>ALGVPFFSCQRGYKGVWRGDGIMQTTCPCGAQITGHVKNGSMRIVGPRTCSNTWHGTFPINAYTTGPCTPSPAPNYSRALWRVAAEEYVEVTRVGDFHYVTGMTTDNVKCPCQVPAPEFFTEVDGVRLHRYAPACKPLLREEVTFLVGLNQYLVGSQLPCEPEP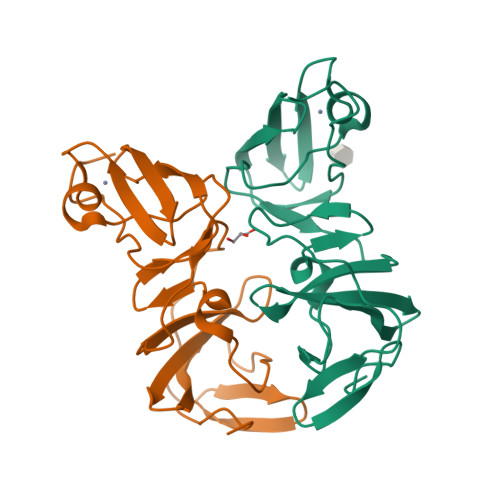DVAVLTSMDDDDK[2x]>[6x]MNSMELLIIKERRIDYDGSAIRSHWAYRNF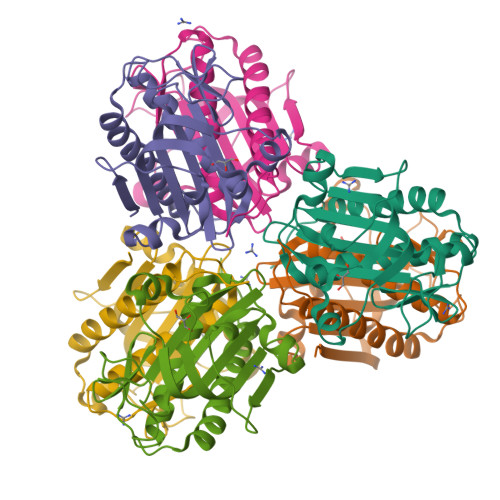GILGDSLVVFRGKCNVKVEEMVDIEDLRLRKEIKGDDMVHYILELFWHPDILLASSLQKLLIARLVELLWNYGIEASRRGDDIYVNGRKLSISIATVSPVSIKIHIGLNVKTVGVPPGVDAIGLEELGIDPTEFMERSAKALVEEIEKVRKDSLKVRWVT In M1 Group A Streptococcus (GAS) strain SF370, pili are comprised of three subunits, Spy0125 (minor tip pilin, also known as “Cpa”), Spy0128 (major pilin), and Spy0130 (minor basal pilin). Most of these pilin domains contain stabilizing intramolecular isopeptide bonds (in Spy0125 these are between Asp595 and Lys297 and between Asn715 and Lys610 of the middle and bottom domains, respectively). Intriguingly, the Spy0125-CTR structure revealed that this top domain contains an internal thioester bond between the side chains of Cys426 and Gln57510. Therefore, the internal thioester in Spy0125 may mediate direct attachment to a host cell factor to promote bacterial adhesion during infection.

To establish whether there are any minor conformational differences between the native and internal thioester variant proteins that could cause the reduction in adhesion (rather than just the loss of the internal thioester), we determined the crystal structure of the Spy0125-CTRCys426Ala variant. The structure shows that the overall fold of the variant is essentially identical to that of the native protein in the P212121 crystal form. The root mean square deviation (rmsd) between the Cα atoms of chain A of the Spy0125-CTRCys426Ala structure and chain B of the native is 0.65 Å. The Spy0125-CTRCys426Ala structure displays the same overall secondary structural elements, with slight differences only apparent in flexible loop regions. The electron density defining the position of Ala426 and Gln575 shows no link between these side chains, as expected. A small reorientation of the side chain of Gln575 results in a new hydrogen bond between the Gln575NE2 atom and the carbonyl O of Asn428. Tyr516, that is in close proximity to the internal thioester in the native structure is located in the same orientation, but no longer forms any hydrogen bonding interaction with these residues. The structure reveals that the only consequence of the Cys426Ala mutation on the protein is the removal of the internal thioester. There are no significant rearrangements in the overall protein fold that can explain the ∼75% loss of bacterial binding previously observed in the adhesion assay. Showing that the overall CD spectrum, proteolytic/thermal stability, and crystal structure of Spy0125-CTRCys426Ala are similar to wild-type protein provides additional, albeit indirect, evidence that the internal thioester has another function—most likely in mediating adhesion.

>[2x]MAHHHHHHSSGLEVLFQGPNQPQTTSVLIRKYAIGDYSKLLEGATLQLTGDNVNSFQARVFSSNDIGERIELSDGTYTLTELNSPAGYSIAEPITFKVEAGKVYTIIDGKQIENPNKEIVEPYSVEAYNDFEEFSVLTTQNYAKFYYAKNKNGSSQVVYAFNADLKSPPDSEDGGKTMTPDFTTGEVKYTHIAGRDLFKYTVKPRDTDPDTFLKHIKKVIEKGYREKGQAIEYSGLTETQLRAATQLAIYYFTDSAELDKDKLKDYHGFGDMNDSTLAVAKILVEYAQDSNPPQLTDLDFFIPNNNKYQSLIGTQWHPEDLVDIIRMEDKKEVIPVTHNLTLRKTVTGLAGDRTKDFHFEIELKNNKQELLSQTVKTDKTNLEFKDGKATINLKHGESLTLQGLPEGYSYLVKETDSEGYKVKVNSQEVANATVSKTGITSDETLAFENNKEPVVPT1-(3-carbamimidoylbenzyl)-N-(3,5-dichlorobenzyl)-4-methyl-1H-indole-2-carboxamide 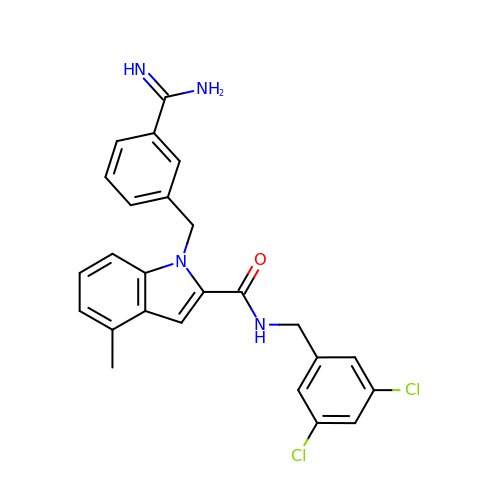| C25 H22 Cl2 N4 O | YAAKSJLUBVPBIM-UHFFFAOYSA-N>[3x]MFEARLVQGSILKKVLEALKDLINEACW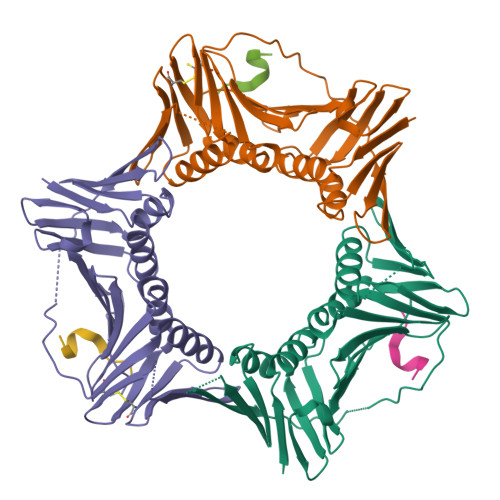DISSSGVNLQSMDSSHVSLVQLTLRSEGFDTYRCDRNLAMGVNLTSMSKILKCAGNEDIITLRAEDNADTLALVFEAPNQEKVSDYEMKLMDLDVEQLGIPEQEYSCVVKMPSGEFARICRDLSHIGDAVVISCAKDGVKFSASGELGNGNIKLSQTSNVDKEEEAVTIEMNEPVQLTFALRYLNFFTKATPLSSTVTLSMSADVPLVVEYKIADMGHLKYYLAPKIEDEE;>[3x]SQRCIPEFF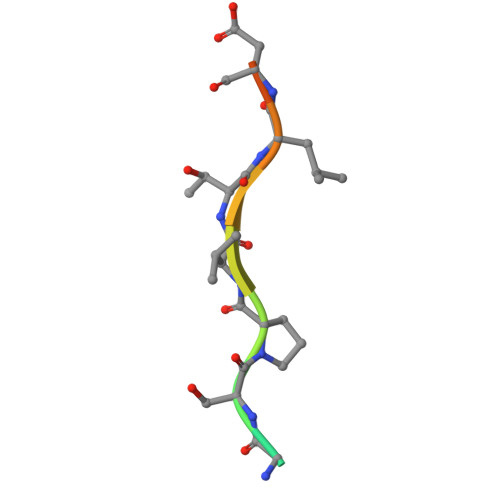> LPEGSPVTLDLRY>[3x]GSAMASMKVYITYGTADFLKTIVKKHPSENILLMQGQENAILIHETSGDTVFQAPHAYEVIDQVGEIK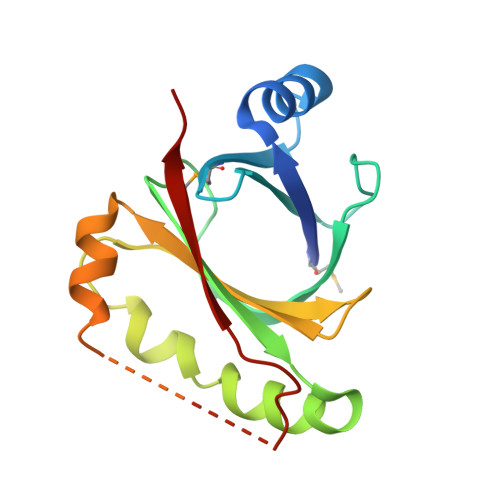HPGFAVLNNIAVTQEGRPLFENKFKNRAGKVENEPGFEAIRVLRPLDSDTYVILTLWETERAFQDWQQSDSYKEAHKKRGTSAGIDTTSIFSRPSYVTTYFAVE> MRRLGVFCRGQRNSPLLTRGIATGGRVTNEDRRWWLVHLECAPDITPGTFIAWLDCCGTHTCKKLIERNIWTIEQVAALDSDQVDELKYREGCLKMDVVWEHARTIITPLRQREVTGGVESELQGRIMELRKKRELERRREEILKERANVSEQREETLRKLRE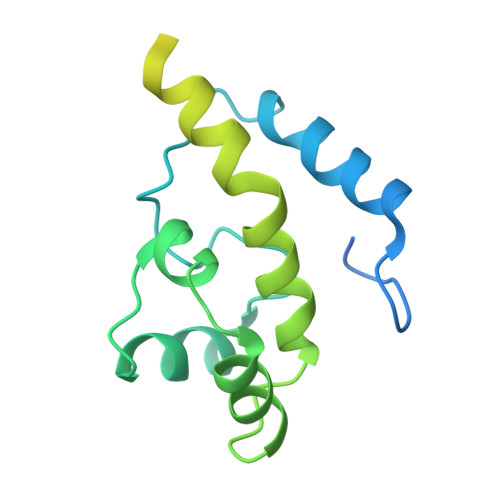AIAAKKAAMXQKKQAASEAYGGSSDGGARKEGAEE> PRGSHMIIETPSKVILFGEHAVVYGYRAISMAIDLTSTIEIKETQEDEIILNLNDLNKSLGLNLNEIKNINPNNFGDFKYC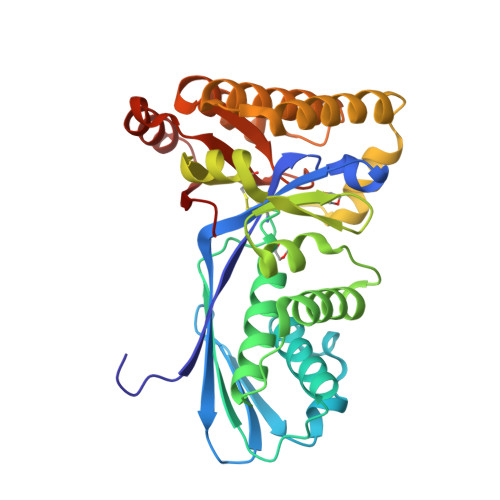LCAIKNTLDYLNIEPKTGFKINISSKIPISCGLGSSASITIGTIKAVSGFYNKELKDDEIAKLGYMVEKEIQGKASITDTSTITYKGILEIKNNKFRKIKGEFEEFLKNCKFLIVYAEKRKKKTAELVNEVAKIENKDEIFKEIDKVIDEALKIKNKEDFGKLMTKNHELLKKLNISTPKLDRIVDIGNRFGFGAKLTGAGGGGCVIILVNEEKEKELLKELNKEDVRIFNCRMMN>MKHTVEVMIPEAEIKARIAELGRQITERYKDSGSDMVLVGLLRGSFMFMADLCREVQVSHEVDFMTASSYGSGMSTTRDVKILKDLDEDIRGKDVLIVEDIIDSGNTLSKVREILSLREPKSLAICT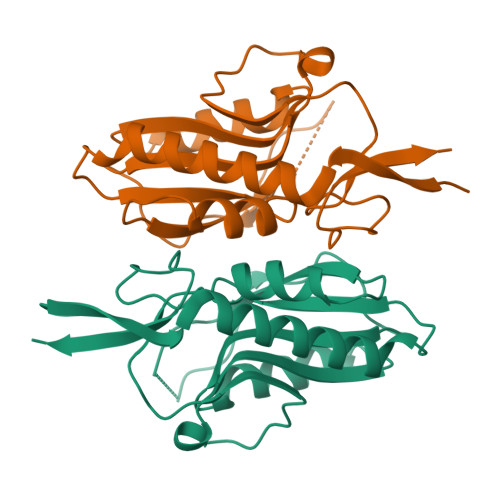LLDKPSRREVNVPVEFIGFSIPDEFVVGYGIDYAQRYRHLPYIGKVILL[2x]>GSEELLDLFNRQVTQEFTASQVYLSASIWFDQNDWEGMAAYMLAESAEEREHGLGFVDFANKRNIPIELQAVPAPVSCAEWSSPEDVWQSILELEQANTRSLLNLAEAASTCHDFAVMAFLNPFHLQQVNAEDKIGSILAKVTDENRTPGLLRSLDVVSFLGPCLFRS[8x]

Ferritin from the marine pennate diatom Pseudo-nitzschia multiseries (PmFTN) plays a key role in sustaining growth in iron-limited ocean environments. Typically formed from 24 subunits arranged as a symmetric, hollow sphere, ferritins take up soluble Fe2+ and catalyze its oxidation, with the resulting Fe3+ being stored as an oxy-hydroxide mineral in its central cavity. The di-iron catalytic ferroxidase center of PmFTN (sites A and B) has a nearby third iron site (site C) in an arrangement typically observed in prokaryotic ferritins. Here we demonstrate that Glu-44, a site C ligand, and Glu-130, a residue that bridges iron bound at sites B and C, limit the rate of post-oxidation reorganization of iron coordination and the rate at which Fe3+ exits the ferroxidase center for storage within the mineral core.

Glu-130, a ligand that can coordinate iron at both site B and site C, was substituted with the non-coordinating residue alanine. Two structures were obtained from E130A PmFTN crystals soaked for 5 min (E130A Fe (5 min)) and overnight (E130A Fe (o.n.)) in aerobic Fe2+ solutions, respectively. The structure obtained from E130A Fe (5 min) has iron bound solely in site A (data not shown). Iron was observed bound to site B and site C in E130A PmFTN, showing that Glu-130 is not essential for iron binding at either site. Remarkably, mineralization in the E130A variant occurred more rapidly, with an initial rate of 40 ± 1 μm Fe2+ min−1, ∼10-fold faster than in wild type PmFTN. In ferritins, such as human H-chain, in which the ferroxidase center functions as a gated site for the transfer of iron into the central cavity, the mineralization rate at lower iron loadings can be interpreted as a measure of the flux of Fe3+ through the center to the central cavity. Consistent with this model, partial regeneration of the initial rapid oxidation phase was observed in E130A PmFTN. Thus, Glu-130 plays a key role in regulating the flux of iron through the ferroxidase center, and we propose that it does this by coordinating Fe3+ at site B such that the rate of exit from the ferroxidase center is limited.The condensin protein complex plays a key role in the structural organization of genomes. Based on their homology to ATP binding cassette (ABC) transmembrane transporters and the Rad50 DNA damage repair protein, the two globular ATPase “head” domains situated at the ends of ∼50-nm-long intra-molecular coiled coils of a heterodimer of condensin’s Smc2 and Smc4 subunits are thought to sandwich a pair of ATP molecules between composite catalytic sites, each composed of Walker A (P loop) and Walker B motifs of one head and a so-called ABC signature motif of the opposite head. Each head domain (hd) can be subdivided into a “RecA”-like lobe that contains the ATP-binding pocket and a “helical” lobe that merges into the coiled coils; they connect the heads to a half-doughnut-shaped “hinge” dimerization domain. Smc2hd and Smc4hd are furthermore connected by their binding to opposite ends of the Brn1Cnd2/NCAPH kleisin subunit (Onn et al., 2007).

In contrast, even the wild-type (WT) version of Ct Smc2hd-Brn1N was unable to bind ATP. This finding is readily explained by the Ct Smc2hd structure, where the more pronounced flexion of the Smc2 helical lobe not only repositions the Q loop but also induces a cascade of structural displacement events that alter the P loop of the ATP-binding pocket into a conformation that is incompatible with nucleotide binding. The Smc2 head fails to bind ATP on its own, presumably because of the deformation of the Smc2 P loop observed in two different crystal forms, but readily binds and hydrolyses ATP when in complex with the Smc4 head. This transition is presumably the consequence of a pronounced reorientation of the Smc2 helical lobe and coiled coil by ∼25° upon head dimerization, which is transmitted via D-loop and adjacent helices to create a P loop conformation that is compatible with nucleotide binding.

> MRVTELIIDGFKSYAVRTVITGWDESFNAVTGLNGSGKSNILDAICFVLGITNMSTVRAQNLQDLIYKRGQAGVTKASVTIVFDNRDKKRSPIGFEEYATISVTRQIVLGGTTKYLINGHRAQQQTVQNLFQSVQLNINNPNFLIMQGRITKVLNMKPAEILAMIEEAAGTRMFEDRKEKALKTMAKKDLKLQEITELLRDEIEPKLEKLRQEKRSGGSGGSMNMIDSVEKKEMSLKHMMKTVLKDKHKIEETIATLDEYKRKALQETWEKVNGDFGQIFNELLPGSFAKLEPPEGKDLTDGLEVKVRLGKVWKQSLTELSGGQRSLIALSLIMALLQFKPAPMYILDEVDAALDLSHTQNIGRLIKTRFKGSQFIVVSLKDGMFQNANRIFRVRFSEGTSVVQALTPADLK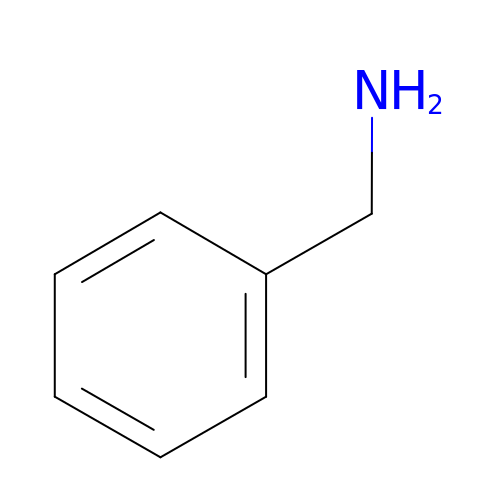BENZYLAMINE | C7 H9 N | WGQKYBSKWIADBV-UHFFFAOYSA-N>[2x]GSMAQIL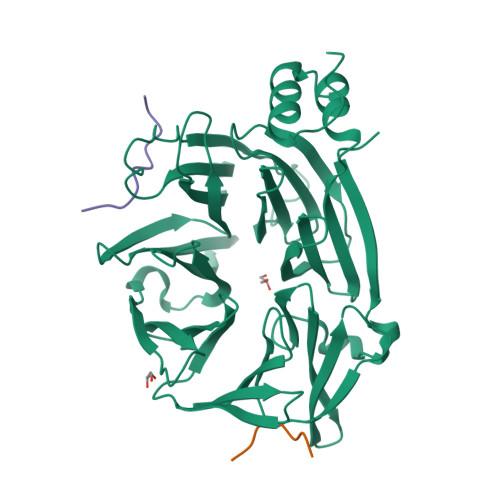PIRFQEHLQLQNLGINPANIGFSTLTMESDKFICIREKVGEQAQVVIIDMNDPSNPIRRPISADSAIMNPASKVIALKAGKTLQIFNIEMKSKMKAHTMTDDVTFWKWISLNTVALVTDNAVYHWSMEGESQPVKMFDRHSSLAGCQIINYRTDAKQKWLLLTGISAQQNRVVGAMQLYSVDRKVSQPIEGHAASFAQFKMEGNAEESTLFCFAVRGQAGGKLHIIEVGTPPTGNQPFPKKAVDVFFPPEAQNDFPVAMQISEKHDVVFLITKYGYIHLYDLETGTCIYMNRISGETIFVTAPHEATAGIIGVNRKGQVLSVCVEEENIIPYITNVLQNPDLALRMAVRNNLAGAEEL;>[4x]ETLLDLDFDP> HHHHHHGDAPGGAHMTAQTVTGAVAAAQLGATLPHEHVIFGYPGYAGDVTLGPFDHAAALASCTETARALLARGIQTVVDATPNGCGRNPAFLREVSEATGLQILCATGFYYEGGGATTYFKFRASLGDAESEIYEMMRTEVTEGIAGTGIRAGVIKLASSRDAITPYEQLFFRAAARVQRETGVPIITHTQEGQQGPQQAELLTSLGADPARIMIGHMDGNTDPAYHRETLRHGVSIAFDRIGLQG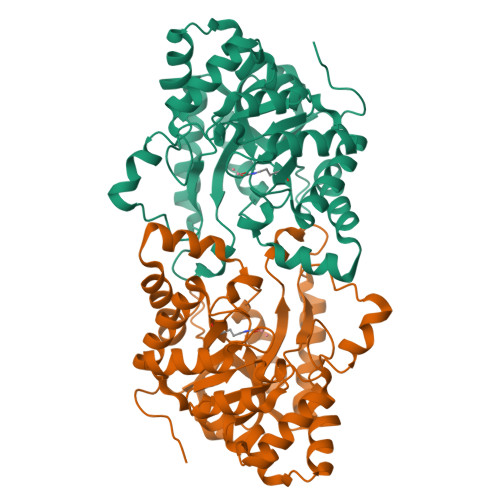MLGTPTDAERLSVLTTLLGEGYADRLLLSHDSIWHWLGRPPAIPEAALPAVKDWHPLHISDDILPDLRRRGITEEQVGQMTVGNPARLFG>MHHHHHHENLYFQGAGAGAGAGAMSELSAIETAAAIAGGSMTALEACDAAIARIEQRDGPINAVVVRDFDRARDAAKAADAEIAAAVRKPLLGVPMTIKESFDIAGLPTSWGFAEHADHIATADSLVVSRLKAAGAVFLGKSNIPVGLADWQSVNPNYGRTNNPHDHSRSAGGSSGGAAAALAAGMVPLEYGSDIGGSIRVPAHFCGVWGLKTTFDAVSLEGHYFPRTDSAKADLSVVGPMARTPADLALALDITSKVPLPQSRIANLSGLRILLLTAHPETVADSATISAVERAAAACEASGATVATSSPDLPDLSALVADYTRMLLVVLARGLAPEGTEPVSLNAWYAMLDDQARMMRAFDRLFESFDAIFCPVLGTTAFAHSDEPDWAKRSLSIDGGIAPFAAQLGWISMATYGGMPALSMPLGADGNGLPINLQIITRNWSDHDAIRIGALVAEALDR[2x]

Here, the ligand‐free crystal structure of UMG‐SP2, a metagenome‐derived urethanase with depolymerization activities, at 2.59 Å resolution, as well as its (co‐)structures bound to a suicide hydrolase inhibitor and a short‐chain carbamate substrate at 2.16 and 2.40 Å resolutions, respectively, is reported. UMG‐SP2 belongs to the amidase signature protein superfamily (AS family), which is characterized by a highly conserved GGSS(S/G)GS motif and can be found in bacteria, archaea, and eukaryotes. SP2 shares the domain architecture of amidases, with an α/β‐fold containing 12 prominent α‐helices, 12 β‐strands, and five larger loops. Structural analysis and molecular dynamics simulations reveal that the flexible loop L3 consisting of residues 219–226 is crucial for regulating the hydrolytic activity of UMG‐SP2.

The crystal structures of wild‐type (WT) UMG‐SP2 (GenBank Accession No. OP972510) were solved in a substrate‐free state (SP2, also used as an interchangeable designation for WT UMG‐SP2 for simplification, 2.59 Å resolution) and a complex with the phenylmethylsulfonyl moiety of the suicide inhibitor PMSF covalently bound to the active site serine 190 (SP2PMS, 2.16 Å resolution). The structure of SP2PMS was solved by molecular replacement (MR), employing the structural coordinates of a structural model of UMG‐SP2 created by AlphaFold2 (AF2). The remainder of the suicide inhibitor PMSF, PMS, bound to the WT SP2 clearly illustrates the topology of the active site architecture, with the amides of residues I187–S190 forming an oxyanion hole and K91, cisS166, and S190 representing the catalytic triad (left inset). The primary active site cavity of SP2 accommodates the phenyl and nitrophenyl moieties of the suicide inhibitor PMSF and BBC, respectively, through a set of hydrophobic residues including W143, W382, L400, L319, and L323. In SP2 and SP2PMS, K224 (part of L3 at the perimeter of the secondary active site cavity) interacts with several water molecules and H215 (as well as S222 in the SP2 structure). These interactions consolidate K224 pointing toward the substrate binding cavity and blocking the secondary active site sterically (right insets). Due to the steric blockage of the active site when empty or partially occupied by PMS, substrate accessibility (in particular for larger molecules) is limited, in contrast to the complex structures with one or two BBC molecules bound. The overall fold of all structures is highly similar, with root mean square deviations (RMSD) of Cα atoms between SP2 and SP2PMS or SP2S190A of 0.2 and 0.25 Å, respectively.>AQEVVGGGDLGPNVLVF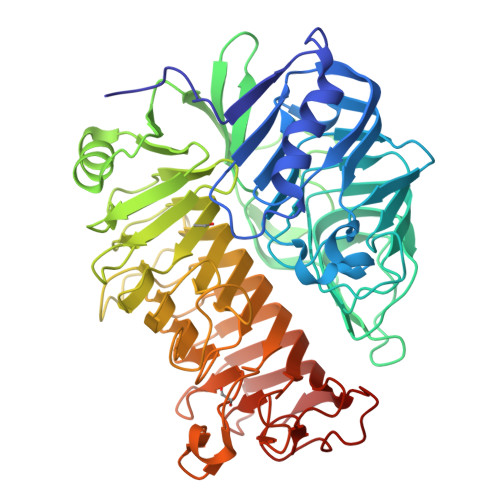DPSTPDIQGKVDEVFRKQESNQFGTDRYALMFKPGTYNDINAQIGFYTSIAGLGLNPDDTTFNGDVTVDAGWFDGNATQNFWRSAENLALNPVNGTNRWAVSQAAPFRRMHVKGGLNLAPDGYGWASGGYIADSKIDGEVGPYSQQQWYTRDSSVGGWGNGVWNMTFSGVEGAPAQSFPEPPYTTLETTPVSREKPFLYLDGDDYKVFVPAKRTNARGTSWGNGTPEGESLPLDQFYVVKPGATAETINAAVDQGLHLLFTPGVYHVDQPIEIDRANTVALGLGLATIIPDNGVTALKVGDVDGVKVAGLLVDAGPVNSETLVEVGSDGASGDHAANPTSLQDVFVRIGGAGPGKATTSIVVNSNDTIIDHTWVWRADHGEGVGWETNRADYGVHVKGDNVLATGLFVEHFNKYDVQWSGENGKTIFYQNAKAYDAPDQAAIQNGDIKGYAAYKVDDSVTTHEGWGMGSYCYFNVNPDIRQQHGFQAPVKPGVKFHDLLVVSLGGKGQYEHVINDIGDPTSGDTTIPSQVVSFP[2x]> MSNKNVNVRKSQEITFCLLAGILMFMAMMVAGRAEAGVALGATRVIYPAGQKQEQLAVTNNDENSTYLIQSWVENADGVKDGRFIVTPPLFAMKGKKENTLRILDATNNQLPQDRESLFWMNVKAIPSMDKSKLTENTLQLAIISRIKLYYRPAKLALPPDQAAEKLRFRRSANSLTLINPTPYYLTVTELNAGTRVLENALVPPMGESTVKLPSDAGSNITYRTINDYGALTPKMTGVME;> MSYLNLRLYQRNTQCLHIRKHRLAGFFVRLFVACAFAAQASLSSAELYFNPRFLADDPQAVADLSRFENGQELPPGTYRVDIYLNNGYMATRDVTFNTGDSEQGIVPCLTRAQLASMGLNTASVAGMNLLADDACVPLTTMVQDATAHLDVGQQRLNLTIPQAFMSNRARGYIPPELWDPGINAGLLNYNFSGNSVQNRIGGNSHYAYLNLQSGLNIGAWRLRDNTTWSYNSSDRSSGSKNKWQHINTWLERDIIPLRSRLTLGDGYTQGDIFDGINFRGAQLASDDNMLPDSQRGFAPVIHGIARGTAQVTIKQNGYDIYNSTVPPGPFTINDIYAAGNSGDLQVTIKEADGSTQIFTVPYSSVPLLQREGHTRYSITAGEYRSGNAQQEKPRFFQSTLLHGLPAGWTIYGGTQLADRYRAFNFGIGKNMGALGALSVDMTQANSTLPDDSQHDGQSVRFLYNKSLNESGTNIQLVGYRYSTSGYFNFADTTYSRMNGYNIETQDGVIQVKPKFTDYYNLAYNKRGKLQLTVTQQLGRTSTLYLSGSHQTYWGTSNVDEQFQAGLNTAFEDINWTLSYSLTKNAWQKGRDQMLALNVNIPFSHWLRSDSKSQWRHASASYSMSHDLNGRMTNLAGVYGTLLEDNNLSYSVQTGYAGGGDGNSGSTGYATLNYRGGYGNANIG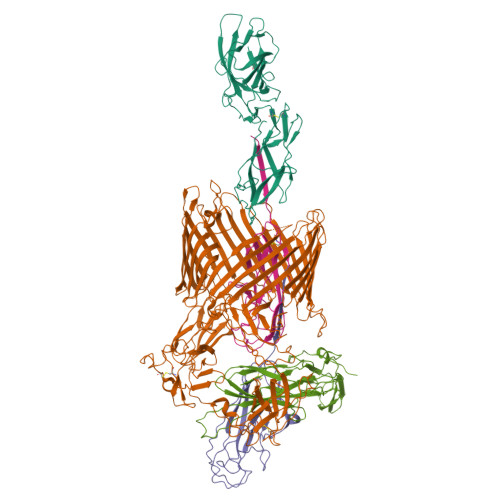YSHSDDIKQLYYGVSGGVLAHANGVTLGQPLNDTVVLVKAPGAKDAKVENQTGVRTDWRGYAVLPYATEYRENRVALDTNTLADNVDLDNAVANVVPTRGAIVRAEFKARVGIKLLMTLTHNNKPLPFGAMVTSESSQSSGIVADNGQVYLSGMPLAGKVQVKWGEEENAHCVANYQLPPESQQQLLTQLSAECRS;> MAADSTITIRGYVRDNGCSVAAESTNFTVDLMENAAKQFNNIGATTPVVPFRILLSPCGNAVSAVKVGFTGVADSHNANLLALENTVSAASGLGIQLLNEQQNQIPLNAPSSALSWTTLTPGKPNTLNFYARLMATQVPVTAGHINATATFTLEYQ;> MAAILALASATIQAADVTITVNGKVVAKPCTVSTTNATVDLGDLYSFSLMSAGAASAWHDVALELTNCPVGTSRVTASFSGAADSTGYYKNQGTAQNIQLELQDDSGNTLNTGATKTVQVDDSSQSAHFPLQVRALTVNGGATQGTIQAVISITYTYS;> MKRVITLFAVLLMGWSVNAWSFACKTANGTAIPIGGGSANVYVNLAPVVNVGQNLVVDLSTQIFCHNDYPETITDYVTLQRGSAYGGVLSNFSGTVKYSGSSYPFPTTSETPRVVYNSRTDKPWPVALYLTPVSSAGGVAIKAGSLIAVLILRQTNNYNSDDFQFVWNIYANNDVVVPTGGCDVSARDVTVTLPDYPGSVPIPLTVYCAKSQNLGYYLSGTTADAGNSIFTNTASFSPAQGVGVQLTRNGTIIPANNTVSLGAVGTSAVSLGLTANYARTGGQVTAGNVQSIIGVTFVYQ> MHVEAMISKHPQARGQTDRSLVQCVEMCFDCAQTCAACADACLGEDKVADLRHCIRLNLDCAEICVAAGSIASRAAGTEESILRTMLQTCAEMCRMCEEECR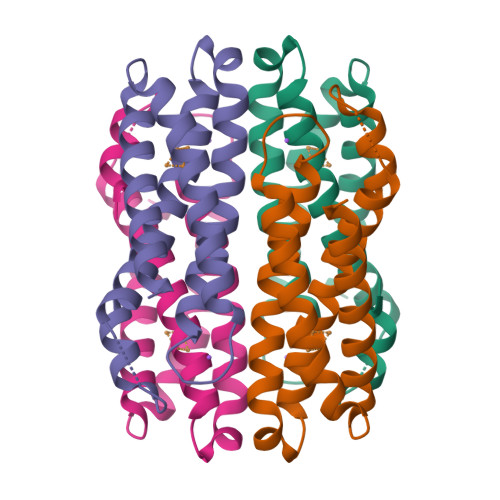RHAGNHEHCRICADVCKECETACRSATGLTH> MREWKIIDSTLREGEQFEKANFSTQDKVEIAKALDEFGIEYIEVTTPVASPQSRKDAEVLASLGLKAKVVTHIQCRLDAAKVAVETGVQGIDLLFGTSKYLRAPHGRDIPRIIEEAKEVIAYIREAAPHVEVRFSAEDTFRSEEQDLLAVYEAVAPYVDRVGLADTVGVATPRQVYALVREVRRVVGPRVDIEFHGHNDTGCAIANAYEAIEAGATHVDTTILGIGERNGITPLGGFLARMYTLQPEYVRRKYKLEMLPELDRMVARMVGVEIPFNNYITGETAFSHKAGMHLKAIYINPEAYE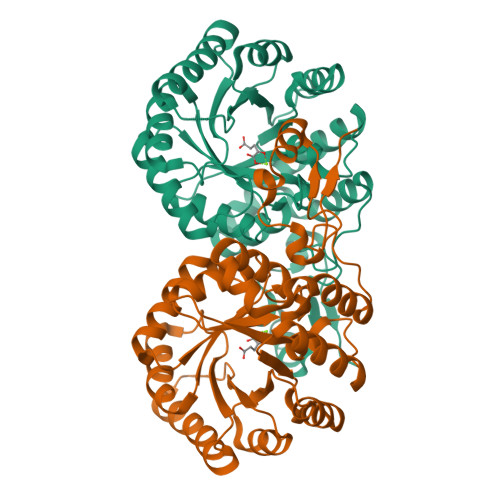PYPPEVFGVKRKLIIASRLTGRHAIKARAEELGLHYGEEELHRVTQHIKALADRGQLTLEELDRILREWITAHHHHHH3,4-dimethoxy-N-[4-(3-nitrophenyl)-1,3-thiazol-2-yl]benzenesulfonamide | C17 H15 N3 O6 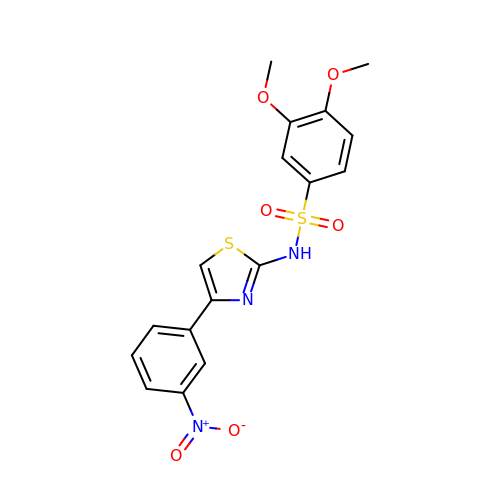S2 | NDPBMCKQJOZAQX-UHFFFAOYSA-N> MINEDFFIYEQLSHKKNLEQKGKNAFDEETEELVRQAKSGYHAFIEGINYDEVTKLDLNSSVAALEDYISIAKEIEKKHKMFNWRSDYAGSIIPEFLYRIVHVATVKAGLKPIFSTRNTIIEISGAAHREGLQIRRKNEDFALGFHEVDVKIASESHRVISLAVACEVKTNIDKNKLNG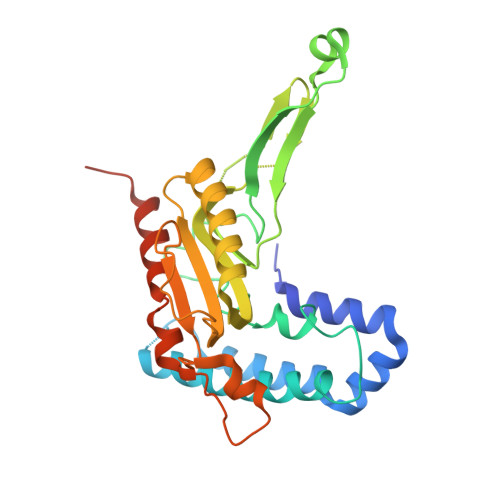LDFSAERMKRTYPGSAYFLITETLDFSPDENHSSGLIDEIYVLRKQVRTKNRVQKAPLCPSVFAELLEDILEISYRASNVKGHVYDRLEGGKLIRV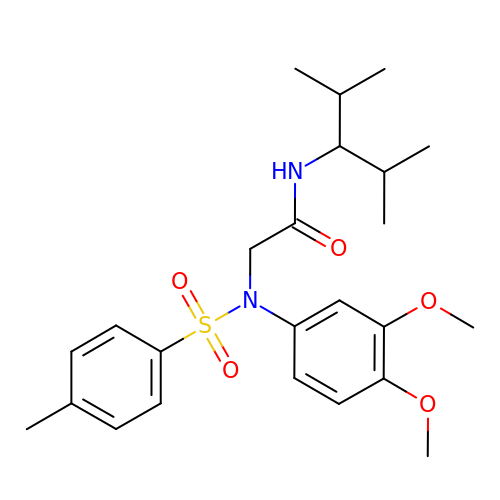2-[(3,4-dimethoxyphenyl)-(4-methylphenyl)sulfonyl-amino]-N-(2,4-dimethylpentan-3-yl)ethanamide | C24 H34 N2 O5 S | WYLSGWZVDHQRNX-UHFFFAOYSA-N>[3x]GTVTTSDGTNIFYKDWGPRDGLPVV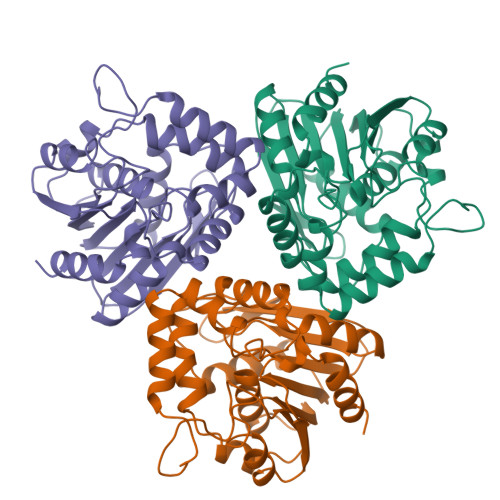FHHGWPLSADDWDNQMLFFLSHGYRVIAHDRRGHGRSDQPSTGHDMDTYAADVAALTEALDLRGAVHIGHSTGGGEVARYVARAEPGRVAKAVLVSAVPPVMVKSDTNPDGLPLEVFDEFRAALAANRAQFYIDVPSGPFYGFNREGATVSQGLIDHWWLQGMMGAANAHYECIAAFSETDFTDDLKRIDVPVLVAHGTDDQVVPYADAAPKSAELLANATLKSYEGLPHGMLSTHPEVLNPDLLAFVKS6-[4-(dimethylamino)butyl]-4-methylpyridin-2-amine 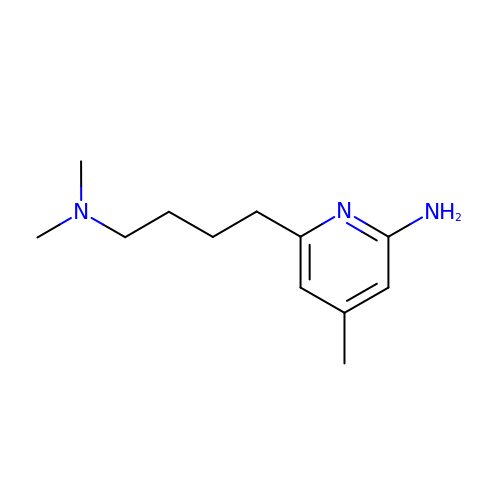| C12 H21 N3 | DBXKFDZMVGIZFJ-UHFFFAOYSA-N> SNAMTDAVLELPAATFDLPLSLSGGTQTTLRAHAGHWLVIYFYPKDSTPGSTTEGLDFNALLPEFDKAGAKILGVSRDSVKSHDNFSAKQGFAFPLVSDGDEA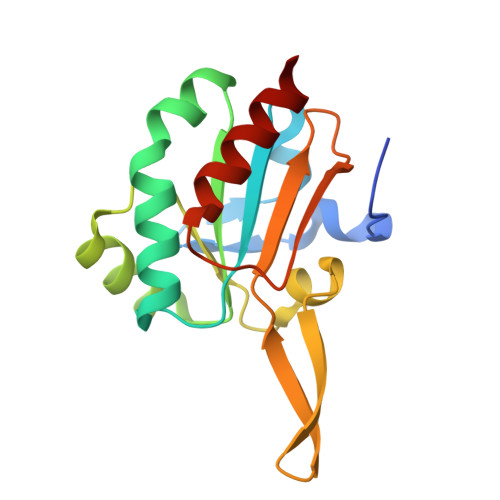LCRAFDVIKEKNMYGKQVLGIERSTFLLSPEGQVVQAWRKVKVAGHADAVLAALKAHAKQ>GPGSGQAIGTLCLIDPSPRLLDLREGRQLNRLSILAEGYLQLRS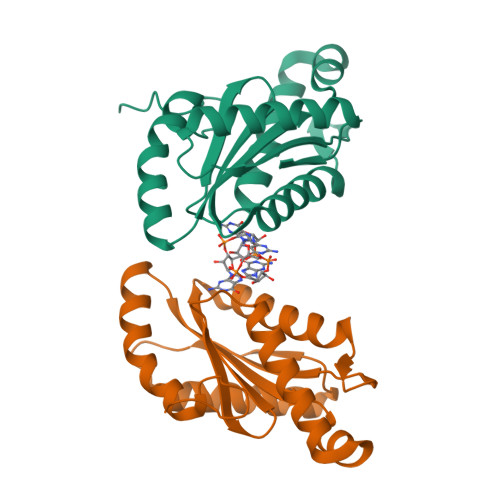LTEHTRFLRQEIDREQRKSLLDPLTQLWNRAGFHALHQHELELARASDQRIGIIYSDIDHFKRINDTLGHRAGDSVLREAASRLRAALRPEDLLARFGGEEFVAMVRVRETTELTMIANRIRELMEATPIDCAGTSVPVTISAGCTLAGSGEEPERALARADAALYDAKRAGRNRVVSV[2x]>MRSRRVDVMDVMNRLILAMDLMNRDDALRVTGEVREYIDTVKIGYPLVLSEGMDIIAEFRKRFGCRIIADFKVADIPETNEKICRATFKAGADAIIVHGFPGADSVRACLNVAEEMGREVFLLTEMSHPGAEMFIQGAADEIARMGVDLGVKNYVGPSTRPERLSRLREIIGQDSFLISPGV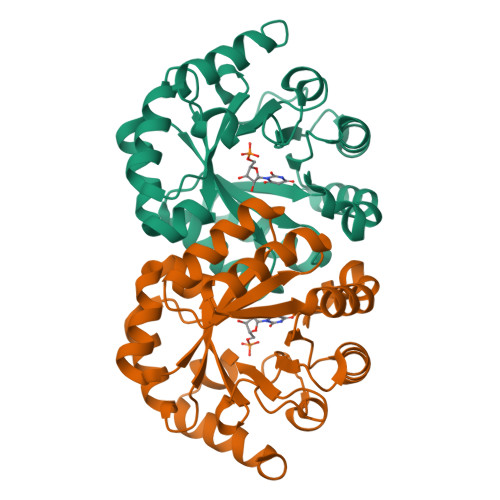GAQGGDPGETLRFADAIIVGASIYLADNPAAAAAGIIESIKDLLNP[2x]> GSFTPVAPIFISLEDVLLNGQLIDFAIDPSGVKFLEANYPLDSEDQIRKAVFEKFTESTTLFVGLCHSRNGNFIVQKLVELATPAEQRELLRQMIDGGLLAMCKDKFACRVVQLALQKFDHSNVFQLIQELSTFDLAAMCTDQISIHVIQRVVKQLPVDMWTFFVHFLSSGDSLMAVCQDKYGCRLVQQVIDRLAENPKLPCFKFRIQLLHSLMTCIVRNCYRLSSNEFANYVIQYVIKSSGIMEMYRDTIIDKCLLRNLLSMSQDKYASHVIEGAFLFAPPALLHEMMEEIFSGYVKDVESNRDA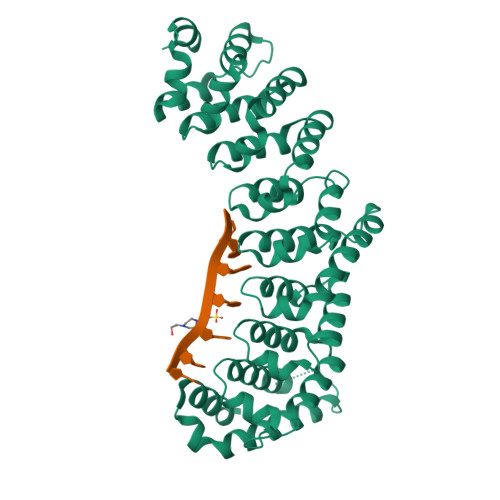LDILLFHQYGNYVVQQMISICTAALIGKEERELPPAILLLYSGWYEKMKQRVLQHASRLERFSSGKKIIDSVMRHG>GGMTAFSTLNVLPPAQLTNLNELGYLTMTPVQAAALPAILAGKDVRVQAKTGSGKTAAFGLGLLQQIDASLFQTQALVLCPTRELADQVAGELRRLARFLPNTKILTLCGGQPFGMQRDSLQHAPHIIVATPGRLLDHLQKGTVSLDALNTLVMDEADRMLDMGFSDAIDDVIRFAPASRQTLLFSATWPEAIAAISGRVQRDPLAIEIDSTDALPPIEQQFYETSSKGKIPLLQRLLSLHQPSSCVVFCNTKKDCQAVCDALNEVGQSALSLHGDLEQRDRDQTLVRFANGSARVLVATDVAARGLDIKSLELVVNFELAWDPEVHVHRIGRTARAGNSGLAISF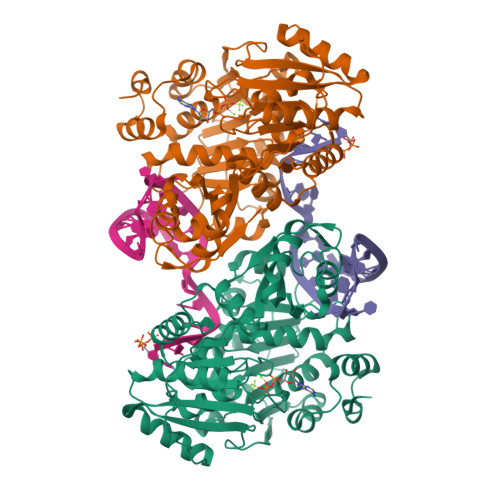CAPEEAQRANIISDMLQIKLNWQTPPANSSIATLEAEMATLCIDGGKKAKMRPGDVLGALTGDIGLDGADIGKIAVHPAHVYVAVRQAVAHKAWKQLQGGKIKGKTCRVRLLK[6x]> MGHHHHHHHHHHSSGHIEGRHMFSKNAVKLHATPPSVAAPPTGAPEVAAERLEPRVEEKDGYWILKEQFRKGINPQEKVKIEKEPMKLFMENGIEELAKIPIEEIDQSKLTKDDIDVRLKWLGLFHRRKNQYGRFMMRLKLPNGVTTSAQTRYLASVIRKYGKEGCADITTRQNWQIRGVVLPDVPEILKGLAEVGLTSLQSGMDNVRNPVGNPLAGIDPEEIVDTRPYTNLLSQFITGNSRGNPAVSNLPRKWKPCVVGSHDLYEHPHINDLAYMPATKDGRFGFNLLVGGFFSAKRCDEAIPLDAWVPADDVVPVCRAILEAFRDLGFRGNRQKCRMMWLIDELGVEGFRAEVEKRMPQQQLERASPEDLVQKQWERRDYLGVHPQKQEGYSFIGLHIPVGRVQADDMDELARLADEYGSGEIRLTVEQNIIIPNIETSKIEALLKEPVLSTFSPDPPILMKGLVACTGNQFCGQAIIETKARSLKITEEVQRQVSLTKPVRMHWTGCPNTCAQVQVADIGFMGCLTRDKNGKTVEGADVFL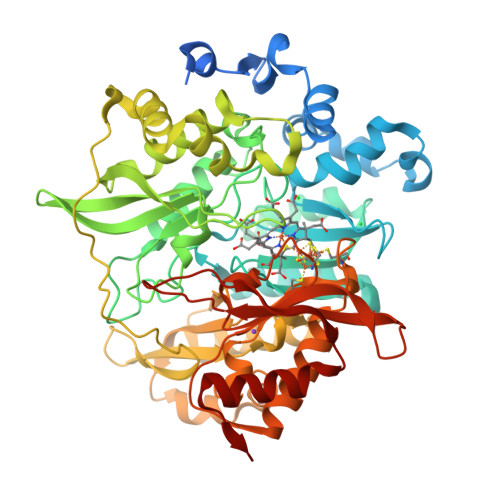GGRIGSDSHLGEVYKKAVPCDDLVPLVVDLLVNNFGAVPR>MRLSMENIMNNPVIGVVMCRNRLKGHATQTLQEKYLNAIIHAGGLPIALPHALAEPSLLEQLLPKLDGIYLPGSPSNVQPHLYGENGDEPDADPGRDLLSMAIINAALERRIPIFAICRGLQELVVATGGSLHRKLCEQPELLEHREDPELPVEQQYA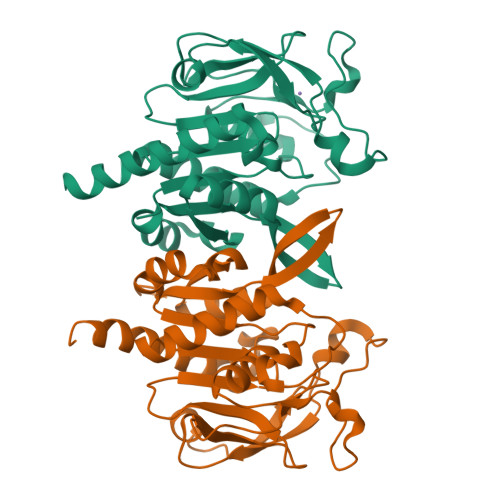PSHEVQVEEGGLLSALLPECSNFWVNSLHGQGAKVVSPRLRVEARSPDGLVEAVSVINHPFALGVQWHPEWNSSEYALSRILFEGFITACQHHIAEKQRL[2x]>GSVESHPVLEKLKAAHSYNPKEFEWNLKSGRVFIIKSYSEDDIHRSIKYSIWCSTEHGNKRLDSAFRCMSSKGPVYLLFSVNGSGHFCGVAEMKSPVDYGTSAGVWSQDKWKGKFDVQWIFVKDVPNNQLRHIRLENNDNKPVTNSRDTQEVPL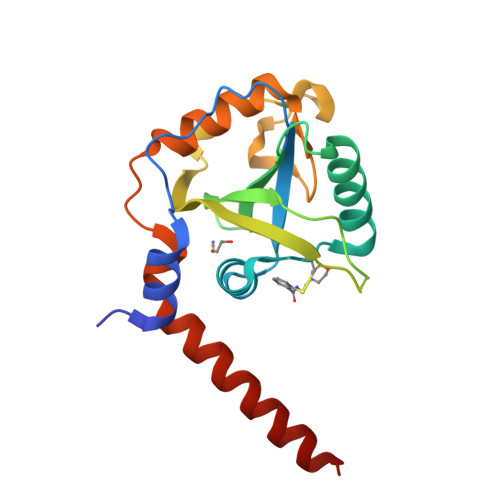EKAKQVLKIISSYKHTTSIFDDFAHYEKRQAVVEVVRKERQSRNKQ[2x]> MGVPAFFRWLTKKYPATVVNANEDRQRDQDGNRVPVDCTQPNPNFQEFDNLYLDMNGIIHPCTHPEDRPAPKNEDEMFALIFEYIDRIYSIVRPRRLLYMAIDGVAPRAKMNQQRSRRFRASKEMAEKEASIEEQRNRLMAEGIAVPPKKKEEAHFDSNCITPGTPFMARLADALRYYIHDRVTNDASWANIEIILSDANVPGEGEHKIMDYVRKQRGNPAHDPNTVHCLCGADADLIMLGIATHEANFNIIREEFVQREKNFIFLRIPVLREYLEKELSMPNLPFKFDVERALDDWVFLCFFVGNDFLPHLPSLEIREGAIDRLIKLYKEMVYQMKGYLTKDGIPELDRVEMIMKGLGRVEDEIFKRRQQDEERFQENQKDDIRLYESGWKDRYYRAKFDVGSDDIEFRHRVAWAYVEGLCWVLRYYYQG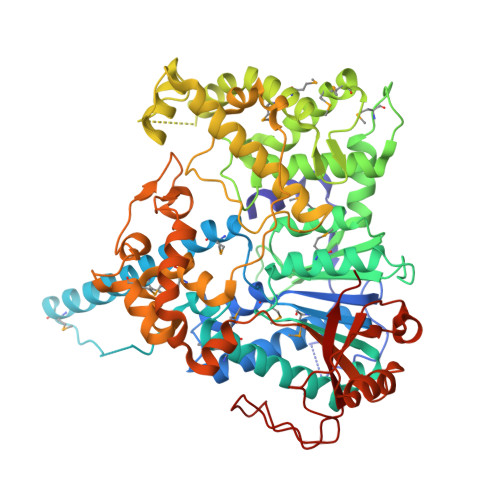CASWDWYFPYHYAPFASDFETVGEFQPDFTRPTKPFNPLEQLMSVFPAASKQHLPVEWQKLMIQDDSPIIDLYPADFRIDLNGKKYAWQGVALLPFVDETRLLATLQSVYPTLTAEEKQRNTRGPNRIFIGRNHKSFEFFQQVAESKSDDLVPLDPTLLNGVSGKIAYDSTATAPGLPFVSPVNHDECQDLPTNCGICVLYEDPE> GFRASRSHSRREEHSGRNGLHHPSPDHFWPRFPDALRPFVPWDQLENEDSSVHISPRQKRDANSSIYKGKKCRMESCFDFTLCKKNGFKVYVYPQQKGEKIAESYQNILAAIEGSRFYTSDPSQACLFVLSLDTLDRDQLSPQYVHNLRSKVQSLHLWNNGRNHLIFNLYSGTWPDYTEDVGFDIGQAMLAKASISTENFRPNFD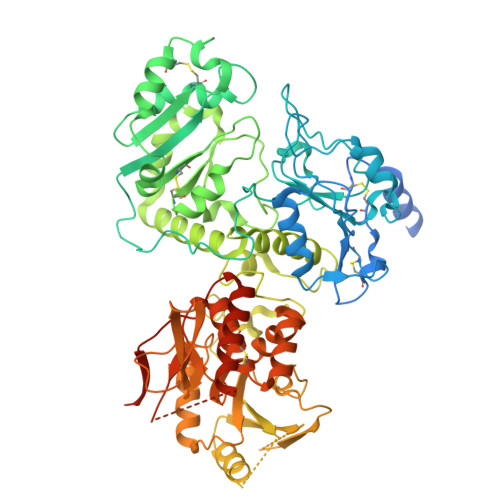VSIPLFSKDHPRTGGERGFLKFNTIPPLRKYMLVFKGKRYLTGIGSDTRNALYHVHNGEDVVLLTTCKHGKDWQKHKDSRCDRDNTEYEKYDYREMLHNATFCLVPRGRRLGSFRFLEALQAACVPVMLSNGWELPFSEVINWNQAAVIGDERLLLQIPSTIRSIHQDKILALRQQTQFLWEAYFSSVEKIVLTTLEIIQDRIFKHISRNSLIWNKHPGGLFVLPQYSSYLGDFPYYYANLGLKPPSKFTAVIHAVTPLVSQSQPVLKLLVAAAKSQYCAQIIVLWNCDKPLPAKHRWPATAVPVVVIEGESKVMSSRFLPYDNIITDAVLSLDEDTVLSTTEVDFAFTVWQSFPERIVGYPARSHFWDNSKERWGYTSKWTNDYSMVLTGAAIYHKYYHYLYSHYLPASLKNMVDQLANCEDILMNFLVSAVTKLPPIKVTQKKQYKETMMGQTSRASRWADPDHFAQRQSCMNTFASWFGYMPLIHSQMRLDPVLFKDQVSILRKKYRDIERL>[2x]MNFKAVIKEVRLKSEHGYTNNFPSGDTLFIELDVEAKEDLQDVVAGILIRDRFGQDIFGINTYLMEKKVELKKGKYLFTFKMPLNLAPGKYTLTVALHKGMDH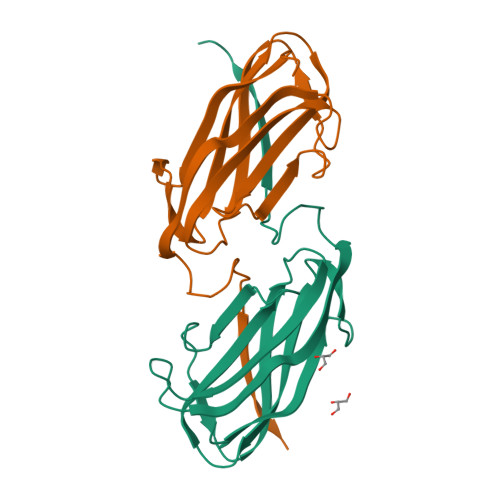AQECYHWIDNVCNFEVNGFKKEQFVGVCYLPTEFNYRKIPKLHHHHHH ALPHA-D-GLUCOPYRANOSYL-2-CARBOXYLIC 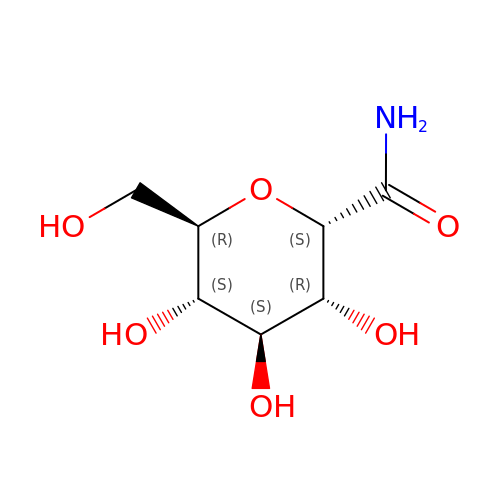ACID AMIDE | C7 H13 N O6 | UKWLGCFJAVEFPE-DVKNGEFBSA-N> SEKEKVEELAQRIREQLPDTELAREAQELADEARKSDDSEALKVVYLALRIVQQLPDTELAREALELAKEAVKSTDSEALKVVELALKIVQQLPDTELAKEALKLAKEAVKSTDSEALKVVELALEIVQQLPDTELAKEALELAEEAVKSTDSEALKVVKLALEIVQQLPDTELAREALELAKEAVKSTDSEALKVVYLALRIVQQLPDTELARLALELAKKAVEMTAQEVLEIARAALKAAQAFPNTELAELMLRLAEVAARVMKELERNDEEIKKSDELDDESLLEDIVELLKEIIKLWKILVEVSDVMLKLIS;> SEKEKVEELAQRIREQLPDTELAREAQELADEARKSDDSEALKVVYLALRIVQQLPDTELAREALELAKEAVKSTDSEALKVVELALKIVQQLPDTELAKEALELAKEAVKSTDSEALKVVELALEIVQQLPDTELAKEALKLAKEAVKSTDSEALKVVYLALRIVQQLPDTELAREALELAKEAVKSTDSEQLEVVRLALEIVQLAPDTRLARAALKLAKEAVKSTDQEELKKVKAILRVASEVLKLEEEAKKSQEEVERLKQEVEKASKAGLDHEGDSRIFKKIHDVVTKQIKVILRLIAVYAELVAIIG;> GSKQKEAIKVYLELLEVHSRVLKALIEQIKLFIELIMEPDEDLADKVRKSSEELKKIIKEVEKILRKVDDILEKVKS

We designed helical heterotrimers with specificity conferred by buried hydrogen bond networks and large aromatic residues to enhance shape complementary packing. Crystal structures of a helical bundle heterotrimer and extended versions, with helical repeat proteins fused to individual subunits, showed all three chains assembling in the designed orientation. We succeeded in determining three high-resolution structures for DHT03: the original base construct, a one-arm version (1arm_A21/B/C) and an elongated two-arm version (2arm_A21/B21/C long). We show that computational design can create cooperative ABC heterotrimers that can assemble as free-standing helical units or as hubs in larger designed assemblies.

Over the core heterotrimer in both structures, the backbones are very similar to that of the base heterotrimer crystal structure, but the resolution is not high enough to determine the state of the designed hydrogen bond networks. The designed junctions between the repeat protein arms and the core bundle are recapitulated in the crystal structures and hold the repeat arms rigidly in close to the designed orientations. Deviations between the crystal structure and design model in the repeat protein arms increase with increasing distance from the central bundle due to lever arm effects arising from the compounding of small orientational differences in the structures of the individual repeats. These structures show that the DHTs can serve as rigid interaction hubs in asymmetric assemblies, which have been more difficult to design than symmetric ones. Subsequent two-arm fusions were made by combining the two working one-arm fusions and testing nine more new fusions to chain B while keeping chain A constant. Eight out of the ten designs tested had three equimolar bands by gel; six designs had a distinct heterotrimer SEC peak present with the ABC species detected by nMS; and four had a very good fit to the design model via SAXS (Fig. 3f (row 3), Extended Data Fig. 3 and Supplementary Fig. 1). To test this idea, equimolar amounts of individually purified A, B and C of DHT03_2arm_A21/B21/C were mixed together and annealed to allow these interfaces to reassemble in the presence of all components. A monodisperse SEC peak containing all three chains by nMS was observed at the same elution volume as the co-expressed tricistronic version, indicating successful reconstitution of the heterotrimer from independently expressed proteins.>[2x]SSEELQNKLEDVVIDRNLLILGKILGEGEFGSVMEGNLKQEDGTSLKVAV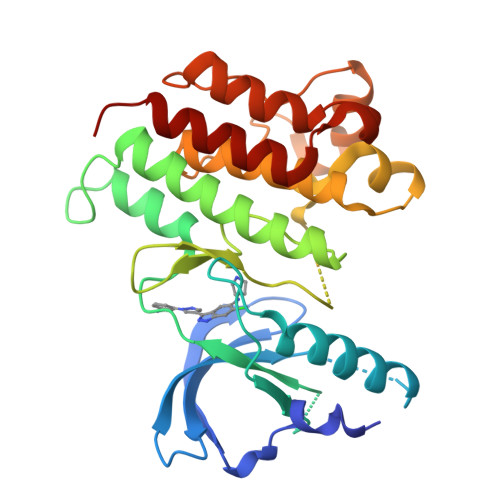KTMKLDNSSQREIEEFLSEAACMKDFSHPNVMRLLGVCIEMSSQGIPKPMVILPFMKYGDLHTYLLYSRLETGPKHIPLQTLLKFMVDIALGMEYLSNRNFLHRDLAARNCMLRDDMTVCVADFGLSKKIYSGDYYRQGRIAKMPVKWIAIESLADRVYTSKSDVWAFGVTMWEIATRGMTPYPGVQNHEMYDYLLHGHRLKQPEDCLDELYEIMYSCWRTDPLDRPTFSVLRLQLEKLLESLPDV>[2x]MMKKADSVPTPAEAALAAQTALAADDSPMGDAARWAMGLLTSSGLPRPEDVAARFIPTFAAAGNFAETVREWRSKGPFTVRAYHPVAHKGWVVLSAPAGVRYILSLTLDSSGLIRILTLKPETVIPDMVTWNDVEETLHTPGVQHSVYAVRLTPDGHEVLHASAPERPMPTGAAYKLYLMRALVAEIEKGTVGWDEILTLTPELRSLPTGDMQDL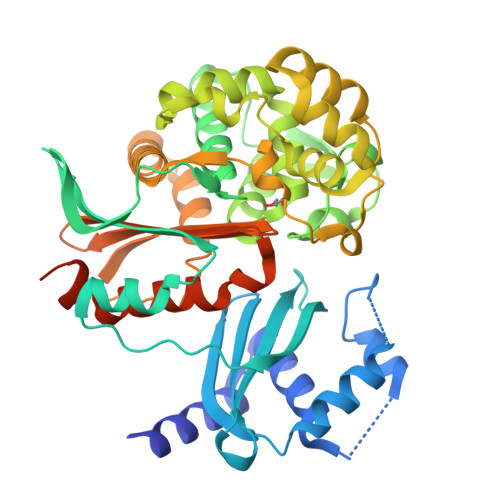PDGTRVTVRETAHKMIALSDNTGADLVADRLGREVVERSLAAAGHHDPSLMRPFLTSHEVFELGWGDPERRAEWVRQDEAGRRELLEKMAGVMTVRGSDLGATVHQLGIDWHMDAFDVVRVLEGLLQDSGRDTSGTVEEILTAYPGLLIDEERWRRVYFKAGSSPGVMMFCWLLQDHAGISYVLVLRQSADEQRLIGDGLFLRGIGAKIIEAEAKLLSSGERRGAGTAAAGDDRASAGEAARR The complex consists of a tripartite ring comprising SMC1, SMC3, and RAD21 (also called SCC1 or Mcd1), which associates with a conserved peripheral fourth subunit that, in human somatic cells, is represented by two paralogs of the Scc3/STAG protein family, STAG1 or STAG2. STAG1/2 HEAT repeat proteins bind to the RAD21 subunit of the core cohesin ring and are required for the dynamic association of the complex with chromatin. The STAG1 protein is composed of HEAT repeats, a tandem repeat structural motif composed of two α helices linked by a short loop. STAG1 and STAG2, therefore, function redundantly in somatic mammalian cells to mediate sister chromatid cohesion, an event essential for cell viability during proliferation.

The STAG1 central region consists of HEAT repeats R6-R14 (residues 459–915), and the structure has been determined both alone and in complex with a 40–amino acid residue RAD21 peptide (spanning residues 356–395) to 2.3 and 3.1 Å, respectively (site VI). As is the case for the N-terminal region, the STAG1 structures are very similar to the STAG2 structure (∼1.4 Å RMSD), with no significant changes observed upon binding to the RAD21 peptide. We have designed constructs of STAG1’s N-terminal and central region encompassing interaction regions I and II, and IV, respectively, and obtained crystal structures in both the presence and absence of the corresponding RAD21 peptides.

>SMSPNGNLIRMLVLFFLESELHEHAAYLVDSLWESSQELLKDWECMTELLLEEPVQGEEAMSDRQESALIELMVCTIRQAAEAHPPVGRGTGKRVLTAKERKTQIDDRNKLTEHFIITLPMLLSKYSADAEKVANLLQIPQYFDLEIYSTGRMEKHLDALLKQIKFVVEKHVESDVLEACSKTYSILCSEEYTIQNRVDIARSQLIDEFVDRFNHSVEDLLQEGEEADDDDIYNVLSTLKRLTSFHNAHDLTKWDLFGNCYRLLKTGIEHGAMPEQIVVQALQCSHYSILWQLVKITDGSPSKEDLLVLRKTVKSFLAVCQQCLSNVNTPVKEQAFMLLCDLLMIFSHQLMTGGREGLQPLVFNPDTGLQSELLSFVMDHVFIDQDEENQSMEGDEEDEANKIEALHKRRNLLAAFSKLIIYDIVDMHAAADIFKHYMKYYNDYGDIIKETLSKTRQID[2x]>[2x]MLNTTFANAKFANPFMNASGVHCMTIEDLEELKASQAGAYITKSSTLEKREGNPLPAYVDLELGSINSMGLPNLGFDYYLDYVLKNQKENAQEGPIFFSIAGMSAAENIAMLKKIQESDFSGITELNLSCPNVPGKPQLAYDFEATEKLLKEVFTFFTKPLGVKLPPYFDLVHFDIMAEILNQFPLTYVNSVNSIGNGLFIDPEAESVVIKPKDG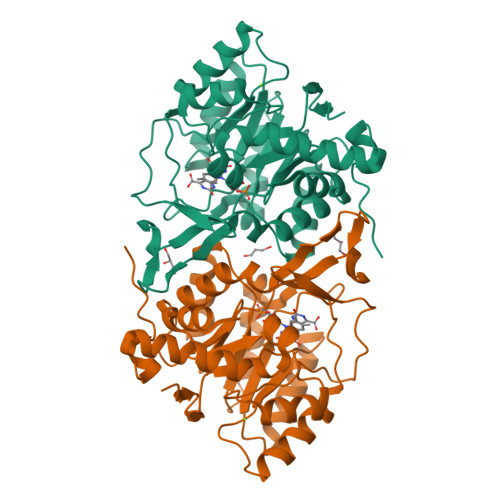FGGIGGAYIKPTALANVRAFYTRLKPEIQIIGTGGIETGQDAFEHLLCGATMLQIGTALHKEGPAIFDRIIKELEEIMNQKGYQSIADFHGKLKSL> GMRLEKDRFSVNLDVKHFSPEELKVKVLGDVIEVHGKHEERQDEHGFISREFHRKY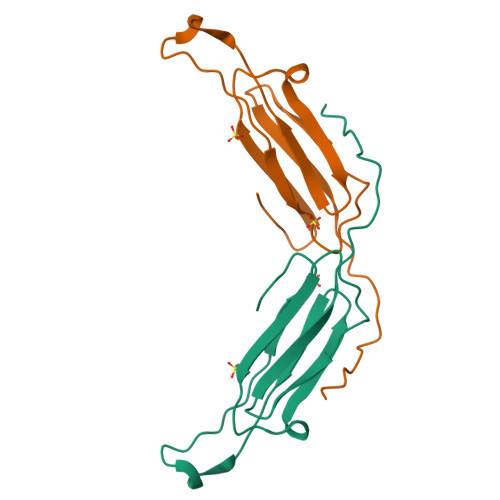RIPADVDPLTITSSLSSDGVLTVNGPRKQVSGPERTIPIT>[4x]MRGSHHHHHHGSMKRVVITGLGIVSSIGNNQQEVLASLREGRSGITFSQELKDSGMRSHVWGNVKLDTTGLIDRKVVRFMSDASIYAFLSMEQAIADAGLSPEAYQN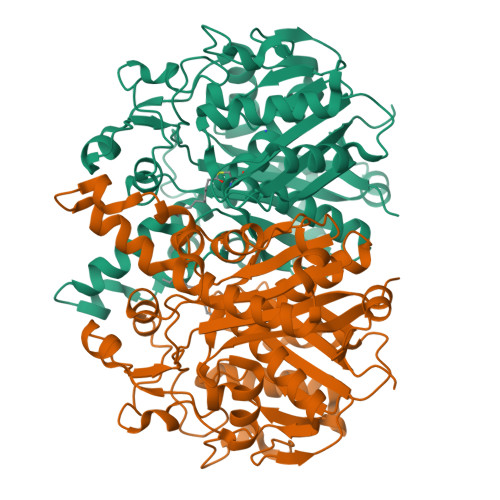NPRVGLIAGSGGGSPRFQVFGADAMRGPRGLKAVGPYVVTKAMASGVSACLATPFKIHGVNYSISSACATSAHCIGNAVEQIQLGKQDIVFAGGGEELCWEMACEFDAMGALSTKYNDTPEKASRTYDAHRDGFVIAGGGGMVVVEELEHALARGAHIYAEIVGYGATSDGADMVAPSGEGAVRCMKMAMHGVDTPIDYLNSHGTSTPVGDVKELAAIREVFGDKSPAISATAAMTGHSLGAAGVQEAIYSLLMLEHGFIAPSINIEELDEQAAGLNIVTETTDRELTTVMSNSFGFGGTNATLVMRKLKD>HHHHHHSEMQDLYPSRQRADAEMRPRLDPVVHSEWTNDAPISARQAAAFDRDGYIVLEDIFSADEVAFLQKAAGNLLADPAALDADTIVTEPQSNEIRSIFEIHAQSPVMARLAADARLADVARFLLGDEVYIHQSRLNYKPGFKGREFYWHSDFETWHVEDGMPRMRALSMSVLLAENTPHNGPLMVIPGSHRTYLTC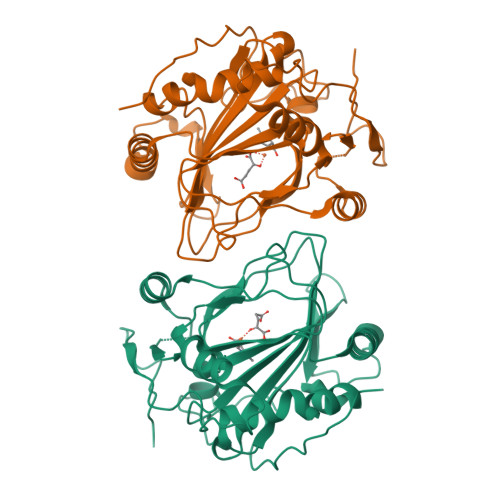VGETPDDHYLSSLKKQEYGVPDEESLAELAHRHGIVAPTGKPGTVILFDCNLMHGSNGNITPFPRANAFLVYNAVSNRLEKPFGVEKPRPWFLARRGEPAALRVERGPLVETVPA[2x]> MGLFDRIKRVVSSNLNDLVNKAEDPEKMLEQAILEMQEDLVQLRQGVAQAIAAQKRSEKQYNDAQNEINKWQRNAQLALQKGDENLARQALERKKTYTDTSAALKASLDTQSTQVETLKRNLIQLESKISEAKTKKEMLKARITTAKAQEQLQGMVRGMNTSSAMSAFERMEEKVLMQESRAQALGEL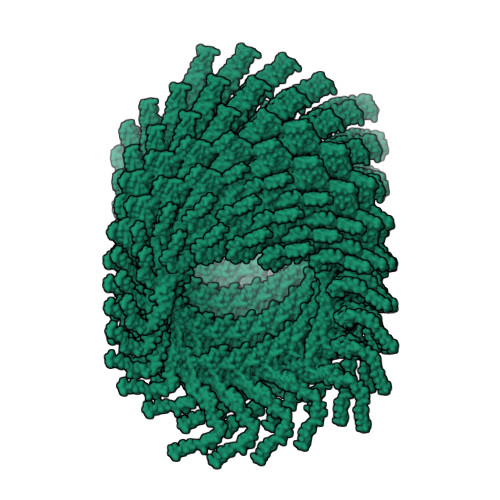AGADLETQFAQLEGGSDVDDELAALKAQMLP AASS is a bifunctional enzyme with an N-terminal lysine-2-oxoglutarate reductase (LOR) domain and a C-terminal saccharopine dehydrogenase (SDH) domain, which are homologous to Saccharomyces cerevisiae LYS1 and LYS9, respectively. The LOR domain catalyses the reductive deamination of L-lysine and 2-oxoglutarate into saccharopine (EC 1.5.1.8), which constitutes the first committed, and possibly rate-limiting, step in lysine degradation. The LOR domain itself consists of two lobes, both Rossman folds with a central beta-sheet with alpha helices on the outside. Moreover, AASS is a unique drug target for inborn errors of metabolism such as glutaric aciduria type 1 that arise from deficiencies downstream in the lysine degradation pathway.

Therefore, to obtain an LOR structure of a protein that maintained catalytic activity, we focused on the longer construct (amino acids 21–470). This initial construct crystallized readily but did not diffract well; therefore, we introduced five surface mutations to induce better packing. The longer construct crystallized in a new space group as a tetramer. (b) Tetrameric structure of the long LOR constructs shown the four monomers assembling into a compact sphere. Each monomer is very similar to the short construct with a root-mean-square deviation (RMSD) of 0.5691 Å2 between the most similar chains. According to the PISA server, the average dimer interface of the longer construct is 1810 Å2 with a predicted ΔG of −6 kcal mol−1. At a structural level, the C-terminus of the longer construct forms an alpha helix that penetrates into the active site of the adjacent monomer. One hypothesis is that the C-terminus interacts with the catalytic residues of an adjacent monomer with the enzyme active only in an oligomeric state. In the structure of the long construct, we see electron density at the interface of these loops from two different monomers that sit between Asp 388 sidechains from each monomer and Glu 373 carbonyl backbones from each monomer. We have assigned this density to a magnesium ion which could help neutralize the negative charge from the aspartates.

>GSHHKAVLAVRREDVNAWERRAPLAPKHIKGITNLGYKVLIQPSNRRAIHDKDYVKAGGILQEDISEACLILGVKRPPAAALMSRKTYAFFSHTIKAQEANMGLLDEILKQEIRLIDYEKMVDHRGVRVVAFGQWAGVAGMINILHGMGLRLLALGHHTPFMHIGMAHNYRNSSQAVQAVRDAGYEISLGLMPKSIGPLTFVFTGTGNVSKGAQAIFNELPCEYVEPHELKEVSQTGDLRKVYGTVLSRHHHLVRKTDAVYDPAEYDKHPERYISRFNTDIAPYTTCLINGIYWAANTPRLLTRQDAQSLLAPGKFSPAGVEGCPALPHKLVAICDISADTGGSIEFMTECTTIEHPFCMYDADQHIIHDSVEGSGILMCSIDNLPAQLPIEATECFGDMLYPYVEEMILSDATQPLESQNFSPVVRDAVITSNGTLPDKYKYIQTLRESRE[4x]> MSNVQTSAEREIVDLSHLAFDCGMLGRLKTVSWTPVIAGDS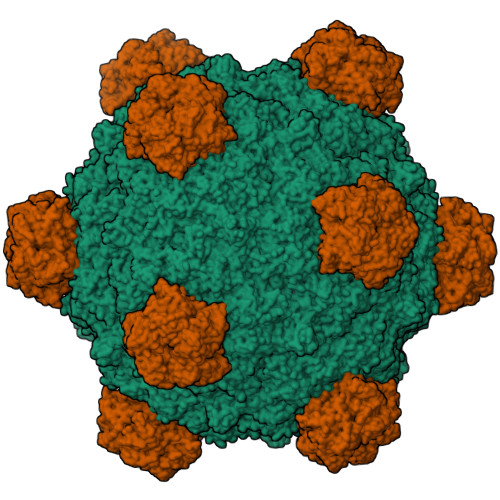FELDAVGALRLSPLRRGLAIDSKVDFFTFYIPHRHVYGDQWIQFMRDGVNAQPLPSVTCNRYPDHAGYVGTIVPANNRIPKFLHQSYLNIYNNYFRAPWMPERTEANPSNLNEDDARYGFRCCHLKNIWSAPLPPETKLAEEMGIESNSIDIMGLQAAYAQLHTEQERTYFMQRYRDVISSFGGSTSYDADNRPLLVMHTDFWASGYDVDGTDQSSLGQFSGRVQQTFKHSVPRFFVPEHGVMMTLALIRFPPISPLEHHYLAGKSQLTYTDLAGDPALIGNLPPREISYRDLFRDGRSGIKIKVAESIWYRTHPDYVNFKYHDLHGFPFLDDAPGTSTGDNLQEAILVRHQDYDACFQSQQLLQWNKQARYNVSVYRHMPTVRDSIMTS;> MYQNFVTKHDTAIQTSRFSVTGNVIPAAPTGNIPVINGGSITAERAVVNLYANMNVSTSSDGSFIVAMKVDTSPTDPNCVISAGVNLSFAGTSYPIVGIVRFESASEQPTSIAGSEVEHYPIEMSVGSGGVCSARDCATVDIHPRTSGNNVFVGVICSSAKWTSGRVIGTIATTQVIHEYQVLQPLK;> MKKARRSPSRRKGARLWYVGGSQF>MASMKVAVLPGDGIGPEVTEAALKVLRALDEAEGLGLAYEVFPFGGAAIDAFGEPFPEPTRKGVEEAEAVLLGSVGGPKWDGLPRKIRPETGLLSLRKSQDLFANLRPAKVFPGLERLSPLKEEIARGVDVLIVRELTGGIYFGEPRGMSEAEAWNTERYSKPEVERVARVAFEAARKRRKHVVSVDKANVLEVGEFWRKTVEEVGRGYPDVALEHQYVDAMAMHLVRSPARFDVVVTGNIFGDILSDLASVLPGSLGLLPSASLGRGTPVFAPVHGSAPDIAGKGIANPTAAILSAAMMLEHAFGLVELARKVEDAVAKALLETPPPD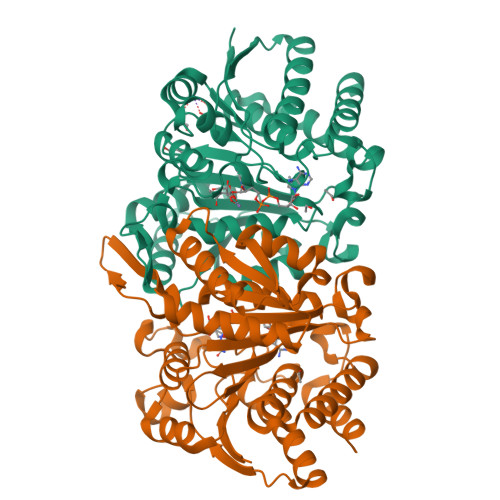LGGSAGTEAFTATVLRHLAAAALEHHHHHH[2x]> MVA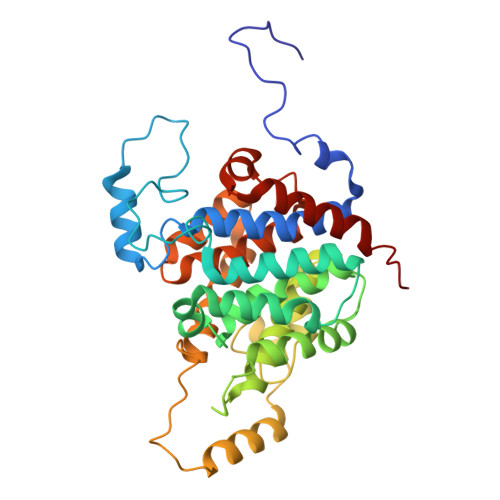KLQHNSAPTTLNFYEKSFQQLSDVQQRQTGLLIGAAVGDAAARALDGYTAEEVAAVAAESGSLQDEDEDPVVFASVTPREHKSGLLRHHSYTFYLFSQLLRVMATSRGDFPVQYVKNEWVATARAHPDCFVREHASLLHVLCITMQLPVIYPWADDSTLREYASGFLEFLTETPAEQAVASREDVYAYTNSVLGVALRCLQSNPDPYRNAAFMAAPGTAHVFPDDLALYCPPALVGSSHSRTEELSETDSETVPLFPARLLESDVRVVRECLVVARGAASFAEGIKAAIHLGGPVCQRSLIVGALLGARMGVRRIPISWLSATYDHVPLVTLALQVAQWSWNPPHH>[48x]MSLGSVLNKVEDADELLKLHDLTEADLALIRKFGQIMVPKLDEYVKHFYDWLRNTPEYEQYFGDAQKLQRVQDSQVRYWKTFFDARIDSAYLKERRDVGEIHARVGLPL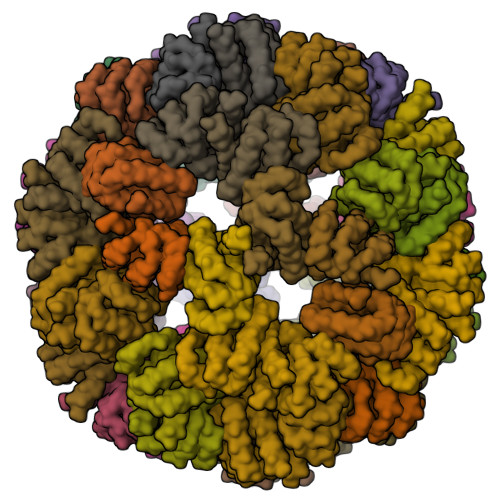PTYFAGMNISMVIFTKRMYDGSLYSDEYSSLVTAFTKLLHLDTTIVVDTYSRLINKRISEQSEALLAMSTPVTMIWQDILMLPIVGIIDSKRAQDIMSAVLNKISENRAKIFIMDISGVAVVDTAVANHFIKITKATKLMGCDCLVSGVSPSIARTMVQLGINVGEVRTNATLRDALENAFKIVGLTVSGLKHFPHE;>[12x]MQSAISISKLQDVLIASVQVDLTESTLRDFSLDLLDAVKSTRAKGVMIELSGVKTLDGESMHSLLDVVKTVEVMGRRCLLVGLRPGVVIGLMDIGIDLASTLCVADLEQGFLYLE>[3x]SSSESLSIIDVASDQNLFQTFIKEWRCKKRFSISLACEKIRSLTSSKTATIGSRFKQASSPQEIPIRDDGFPIKGCDDTLVVGLAVCW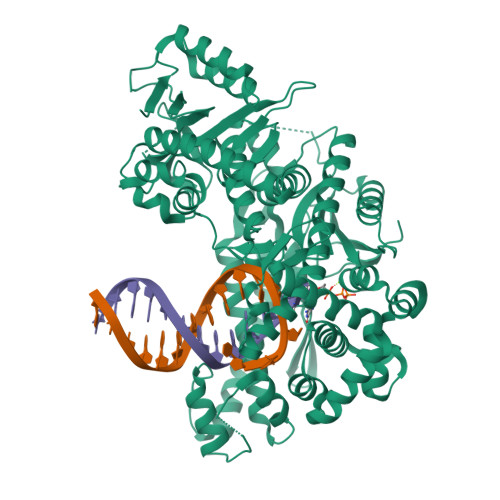GGRDAYYFSLQKEQKHSEISASLVPPSLDPSLTLKDRMWYLQSCLRKESDKECSVVIYDFIQSYKILLLSCGISLEQSYEDPKVACWLLDPDSQEPTLHSIVTSFLPHELPLLEGMETSQGIQSLGLNAGSEHSGRYRASVESILIFNSMNQLNSLLQKENLQDVFRKVEMPSQYCLALLELNGIGFSTAECESQKHIMQAKLDAIETQAYQLAGHSFSFTSSDDIAEVLFLELKLPPNREMKNQGSKKTLGSTRRGIDNGRKLRLGRQFSTSKDVLNKLKALHPLPGLILEWRRITNAITKVVFPLQREKCLNPFLGMERIYPVSQSHTATGRITFTEPNIQNVPRDFEIKMGGMPFSISMRHAFVPFPGGSILAADYSQLELRILAHLSHDRRLIQVLNTGADVFRSIAAEWKMIEPESVGDDLRQQAKQICYGIIYGMGAKSLGEQMGIKENDAACYIDSFKSRYTGINQFMTETVKNCKRDGFVQTILGRRRYLPGIKDNNPYRKAHAERQAINTIVQGSAADIVKIATVNIQKQLETFHSTFKSHGHREGMLQSDQTGLSRKRKLQGMFCPIRGGFFILQLHDELLYEVAEEDVVQVAQIVKNEMESAVKLSVKLKVKVKIGASWGELKDFDV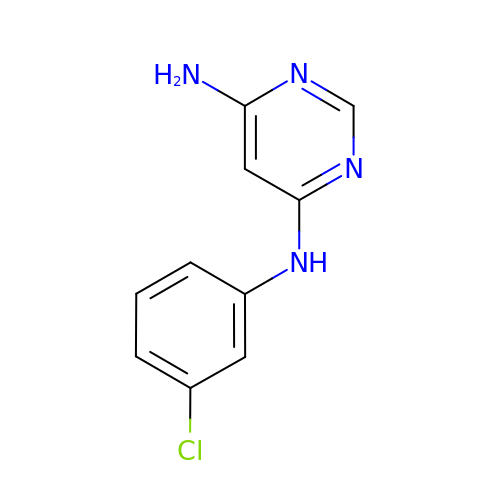N~4~-(3-chlorophenyl)pyrimidine-4,6-diamine | C10 H9 Cl N4 | YEESRFWVWLZFDI-UHFFFAOYSA-N> GVRQYKIHTNLDGTDDKVWDVTNGKVRFYQPSNLGLQSTNNIWQSNGIGVMGTRSITQPQIEFKLETFGESLEENYQLMKDFVNDILSKKFVTLEYQTEIFQVYADLALADVTKTEGYGKNGTFSEKI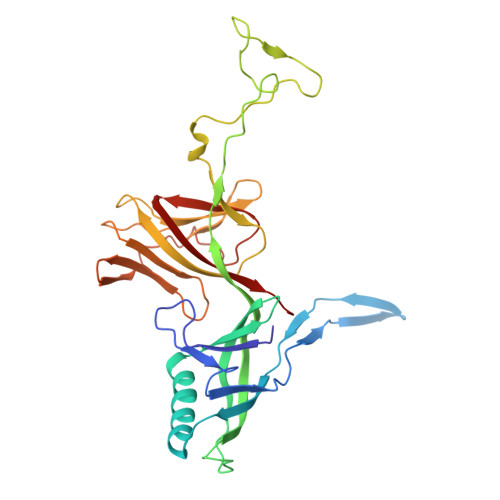TFDIITKWYTYENLTFDKIQNGKVIAGMSKIYGGTAPGNYKYIKGTSYTYYGESDIDRLSRWDIKEEIFSFMGILYPKLPKTPAGVRFLDDIGNEYTAIVFKTEQVQDYILINTDVNDETYQGWKGTTALNLFPVMDFERYRTRIIEKGQMELINLSKAEFKIKRKADFV>SNAPLNRLGHKIYQHSGKWLQETAAEKLNQRDQLINPGHAQVLILGMGRIGTGAYDELRARYGKISLGIEIREEAAQQHRSEGRNVISGDATDPDFWERILDTGHVKLVLLAMPHHQGNQTALEQLQRRNYKGQIAAIAEYPDQLEGLLESGVDAAFNIYSEAGSGFARHVCKQLEP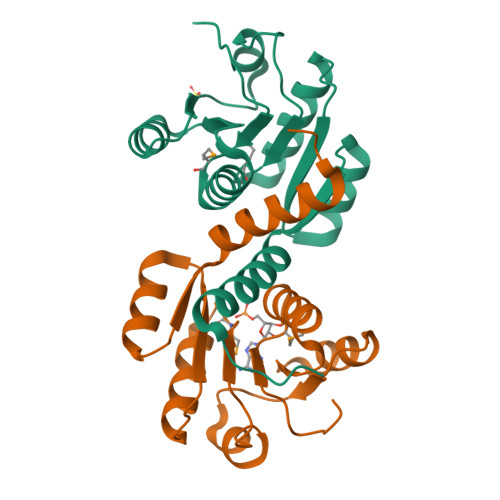QFTSIK[4x]> AAAAA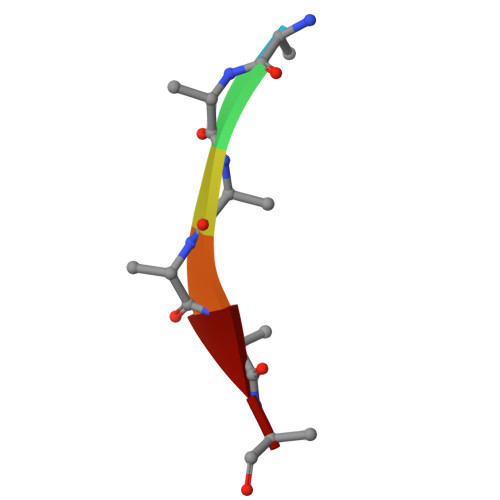A> KAPRKQLA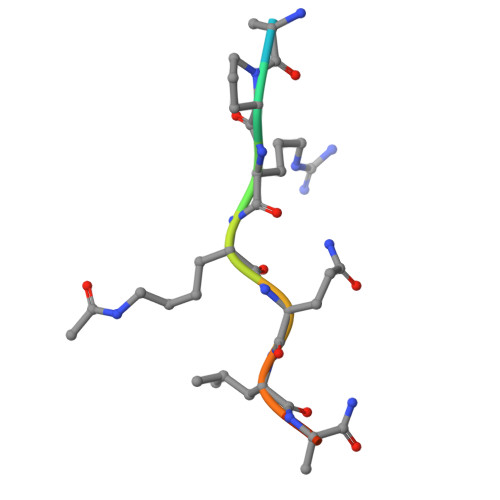TK The loading of ring-shaped, replicative helicases onto DNA constitutes a key event during the initiation of chromosomal DNA replication. In Orc1–5, the AAA+ modules are augmented by a C-terminal HTH domain of the winged-helix (WH) type and co-assemble into a pentameric ring that can exist in both open (active) or closed (autoinhibited) configurations. Structural studies have revealed that the initiator binds DNA in the center of the ORC ring, bending DNA to prepare origins for Mcm2–7 recruitment and loading. To resolve these outstanding questions, we determined cryo-EM structures of DNA-bound Drosophila ORC (DmORC) assemblies in the presence and absence of the co-loader Cdc6.

Importantly, we observe a similar DNA configuration and DNA interactions in a ~3.9 Å resolution cryo-EM structure of a binary DmORC·DNA complex reconstituted in the absence of Cdc6, indicating that Cdc6 binding does not substantially remodel ORC–DNA contacts. The main difference between both structures pertains to the Orc2 WH domain, which is not visible in DmORC·DNA. By contrast, more extensive remodeling is observed in the ORC ring during DNA binding to the initiator when comparing structures of DNA-free, active DmORC and DmORC·DNA. Surprisingly, Cdc6 binding does not remodel ORC–DNA contacts or alter DmORC’s ATPase activity, nor does it induce major conformational changes in the ORC ring apart from providing an interaction surface for the Orc2 WH domain, which is flexible in Cdc6′s absence. These findings indicate that Cdc6 predominantly has a structural role during Mcm2–7 loading. As Cdc6 binding to DmORC·DNA does not alter how the initiator engages DNA, these binding assays report on ORC–DNA contacts in both the binary and ternary complexes. By comparison, the β-hairpin of Orc3 and the WH-helix 2 of Orc5 only moderately contribute to stabilizing DmORC on DNA, with triple mutations of basic residues (Orc3K710A/R711A/K712A or Orc5K341A/K344A/R345A) decreasing DmORC’s affinity for DNA by only 2–3 fold. These biochemical data are congruent with the multivalent protein/DNA interactions observed in both DmORC·DNA and DmORC·DNA·Cdc6 cryo-EM structures, and also uncover the B-loop in Orc1 as a DNA binding element that is essential for high-affinity interactions of DmORC with DNA in the absence and presence of Cdc6.

> SNAPRRSIHLSNIVEQRVFEDDEIISTPKRGRSKKTVQDNDEDYSPKKSVQKTPTRTRRSSTTTKTATTPSKGITTATATPMTPSQKMKKIRAGELSPSMQQRTDLPAKDSSKSELQLAREQLHVSVVPKSLPCREREFENIYAFLEGKIQDQCGGCMYVSGVPGTGKTATVTGVIRTLQRMAKQNELPAFEYLEINGMRLTEPRQAYVQIYKQLTGKTVSWEQAHALLEKRFTTPAPRRVTTVLLVDELDILCNRRQDVVYNLLDWPTKSAAKLVVVTIANTMDLPERLLMGKVTSRLGLTRLTFQPYSHKQLQEIVTARLGGSETFKGEAVQLVARKVAAVSGDARRALDICRRATEIADTAAVKCVTMLHVQQALAEMIASAKVQAIRNCSRMEQIFLQAIAAEVTRTGVEETTFMGVYQQVETIAAFMGVTFPPPGRALRLCSKLGAERLIISEHSRNDLFQKILLNVSADDIHYALRVEEMVN;> MSASNKGGYKTPRKENLMSIENLTNSEEESEDLNTAMVGNAVESQPKVTSRRSTRRPSPTKKYQAYQKESNGKGQEERIVVNYVEMSDERSSDAEDQEEEESIEESENAARPAAKDLHLIQSEYNVAGTSMFGFNTPKKRDAMALAALNATPCTPKTPKTPRLGVKTPDTKRKKSMDQPKTPAHVRTRVKKQIAKIVADSDEDFSGDESDFRPSDEESSSSSSSSDAGNSSDNDAADDEPKTPSRARRAIVVPVLPKTPSAARLRQSARAKKSNEFVPESDGYFHSHASSKILTSDHTLDRLKNPRLAADRVFSLLSEIKTSAEHEGSINAIMEEYRSYFPKWMCILNEGFNILLYGLGSKHQLLQSFHREVLHKQTVLVVNGFFPSLTIKDMLDSITSDILDAGISPANPHEAVDMIEEEFALIPETHLFLIVHNLDGAMLRNVKAQAILSRLARIPNIHLLASIDHINTPLLWDQGKLCSFNFSWWDCTTMLPYTNETAFENSLLVQNSGELALSSMRSVFSSLTTNSRGIYMLIVKYQLKNKGNATYQGMPFRDLYSSCREAFLVSSDLALRAQLTEFLDHKLVKSKRSVDGSEQLTIPIDGALLQQFLEEQEKK;> MDPTISVSKGCFVYKNGATRAGKKAASKRKRPAAESSSLLGKEVVQQPFYEEYRKAWNQINDHIADLQHRSYARTLEQLVDFVVGQAERDTPDEVLPTAALLTGINQPDHLSQFTALTQRLHAQRAAMVCVLQSRDCATLKAAVETLVFGLVEDNAEVEQMEDEDEDEDGAERDRKRLRRSQCTMKQLKSWYTNNFDSEQKRRQLVVILPDFECFNASVLQDLILILSAHCGSLPFVLVLGVATAMTAVHGTLPYHVSSKIRLRVFQTQAAPTGLNEVLDKVLLSPKYAFHLSGKTFKFLTHIFLYYDFSIHGFIQGFKYCLMEHFFGGNAFALCTDYSKALGRIKQLTHEDMETIRRLPSFRPYVEQINDCKRIIAVLTDDDYLKKKLPQLLRDCLLHFLLFRCSLEFLTELVGDLPRCPLGKLRRELYVNCLNRAIISTPEYKECLQMLSFLSKDEFVAKVNRALERTEQFLVEEIAPLELGEACTAVLRPKLEAIRLAVDEVVKATMATITTTSPNETRQATDHLTPVASRQELKDQLLQRSKEDKMRHQLNTPTTQFGRALQKTLQLIETQIVQDHLRALQDAPPIHELFVFSDIATVRRNIIGAPRAALHTALNNPHFYMQCKCCELQDQSLLVGTLPDLSVVYKLHLECGRMINLFDWLQAFRSVVSDSDHEEVAQEQIDPQIQARFTRAVAELQFLGYIKMSKRKTDHATRLTW;> SNAMPEADRELVSIRRFLKERLQRDYTTLRGYAKERSNVRLLLQRTAEMGESNSLLLLGPRGSGKTTLINSVLADLLPNKSFGENTLIVHLDGNLHTDDRVALKSITVQMQLENAADGKVFGSFAENLAFLLQCLKAGGKHSKSVIFILEEFDLFCAHHNQTLLYNLFDVSQSAQAPICVLGVTCRLDVIELLEKRVKSRFSHRQVFLFPSLRRFEDYVDLCRDLLSLPTGNSLLLAAEKIYNLQNIQSGALYFSRNHFDPGEYGFSPRLRDAWNKQICKVLATQQARSTLQALHDFDISEAYLKNFLFRLVAHLRPQSPHITAEKMAAVGSQFEGDDKIELLCGLSVLELCLIIAIKHHSQIYDRDSFNFEIIYARFSKFAKVSTTMQAVERSIVLKAFEHLRIAELIMPLTGGAGGGVGKVQKEFEMHKLALTYSQIHHCMQRYQALPTEVAQWAQSSLI;> MEAICSSLEPLFPCREAAIETLGELIGDSSETYPSAIYLFGHSGTGKTALTRAFLKECGKRQNVRTAHLNAIECYTTKIMLEILLDSLAPDQGDALKVDNMLDFVEQLRRQAATRVEDQGFLIAVDNAERLRDMDANVLPVLLRLQELTNLNLCVILLSQLPFEKFYNKTGLSEIVCLHLAQYNKAETQRILGSDFQQVRNQLLEQFAQDKKRLEICQEAVTEDFYNNYLNLFLSVFYKACRDVPELQLTARKCLSTYLEPVLDGTVDATDISRLWRHIAGPLRSALTQIYMRIEKPAEEVEDFTAIEDQSVRKLAQSLELPYYAKFLLIAAFLASHNAAKQDKRLFVKHHGKQRKRMQTVNARAKTTEKMSTTLGPKSFSIDRLLAIFYAILEEKVGLTCNLLSQISTLVHLNLLSFVSGEQNIMEGSARLQCTIGLEFVLQIGKVVGFNVRQYLCDFM;> MTTLIEQLITKMGLREEPNVLEKTTELVRLLELRSTNVPLQINEYGKIVLCADLASCMIGIAFDKEQALKLSGLRKSQYLNNKRMFEKLLDLNKLASVNDICVQLGLNEVARKAEELMTLFKGVAATEDMGTDTSHPQYATMAVFQACRLLKKKVSKSKLMPFSNLRPSQFQLLEQQWERMIAKHHKESKVPSSTDMEGKLKENQNENIKGHEAKKAHKPPPEDYEIWKARMLAKAQAKLKELEASQSHMDSQLLEA Two enzymes, peptidylglycine α-hydroxylating monooxygenase (PHM; EC 1.14.17.3) and peptidyl-α-hydroxyglycine α-amidating lyase (PAL; EC 4.3.2.5) working sequentially are the only proteins known to catalyze this reaction. PHM, a two Cu enzyme, catalyzes the stereospecific hydroxylation of the glycine Cα of peptidylglycine substrates. The two copper atoms in PHM, CuH, and CuM (located in the N- and C-subdomains, respectively), each use a single reducing equivalent from ascorbate to catalyze the reduction of molecular oxygen for the hydroxylation of the Cα of glycine at the carboxy-terminus of the peptide substrate. Crystallographic data on apo wild-type PHM and on several crystal forms of three CuH mutants (H107A, H108A, and H172A) presented here show that the copper ions are required not only for the catalytic steps but also for substrate binding and for locking the overall conformation of PHM in a configuration that is catalytically active.

Inclusion of 1–3 mM citrate, which produced crystals (H107A-PHM-cit) that diffracted to higher resolution, had unexpected effects on the structure of H107A-PHM and provided information about alternative conformations that can be adopted by this mutant. H107A-PHM-cit has two molecules in the asymmetric unit. Interestingly, the copper sites of these two molecules (A and D) present in the same unit cell have very different configurations, probably because citrate is only present in one of the molecules (molecule D). In molecule A, copper binds at the CuH site despite the absence of His 107 by retaining the coordination with His 108 and His 172 and adding two water molecules as ligands. Even though molecule A does not have a bound citrate, it shows a change in the conformation of the loop containing residues 126 to 130 that brings Glu 128 into the proximity of the CuM site. Molecule D, in contrast, has no copper at the CuH site and contains a bound citrate that bridges the two remaining histidines of the copperless CuH site to the CuM site. Citrate binds close to the empty site of CuH and interacts directly with H108 and H172; the carboxylate of the citrate partially occupies the space that in wild-type PHM forms the peptide binding site. Loss of coordination by H107 allows the CuH site to adopt a tetrahedral coordination by the inclusion of two water molecules, implying that square planar geometry at the H site is destabilized relative to the tetrahedral alternative. This observation strengthens the case for a functional requirement for a non-reactive open coordination site in CuH that allows electron transfer but prevents binding of small molecules that could modify the electrochemical potential of the copper.

>[2x]NECLGTIGPVTPLDASDFALDIRMPGVTPKESDTYFCMSMRLPVDEEAFVIDFKPRASMDTVAHMLLFGCNMPSSTGSYWFCDEGTCTDKANILYAWARNAPPTRLPKGVGFRVGGETGSKYFVLQVHYGDISAFRDNHKDCSGVSVHLTRVPQPLIAGMYLMMSVDTVIPPGEKVVNADISCQYKMYPMHVFAYRVHTHHLGKVVSGYRVRNGQWTLIGRQNPQLPQAFYPVEHPVDVTFGDILAARCVFTGEGRTEATHIGGTSSDEMCNLYIMYYMEAKYALSFMTCTKNVAPDMFRTIPAEANIPIPV>MAHHHHHHMDALDLLLNRRSASRLAEPAPAGEQLENILRAGLRAPDHGTLQPWRFFIIADDGRERFSQLLEKGAREAGQDEKGIEKARNAPFRAPLIITVVARCEDHPKVPRWEQEMSAGCAVMAMQMAALAQGFNGIWRSGALTESPVVRAGFE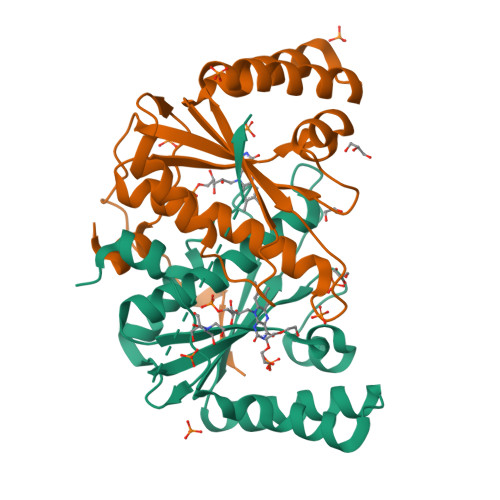CREQDKIVGFLYLGTPQLKASTTIALPDTAPFVTRF[2x]>MGACPPKAKGPWAQLQKLLISWPVGEQDWEQYRDRVNMLQQERIRDSPLLQAAKENDLRLLKILLLNQSCDFQQRGAVGETALHVAALYDNLEAATLLMEAAPELAKEPALCEPFVGQTALHIAVMNQNLNLVRALLARGASVSARATGAAFRRSPHNLIYYGEHPLSFAACVGSEEIVRLLIEHGADIRAQDSLGNTVLHILILQPNKTFACQMYNLLLSYDEHSDHLQSLELVPNHQGLTPFKLAGVEGNTVMFQHLMQKRKHVQWTCGPLTSTLYDLTEIDSWGEELSFLELVVSSKKREARQILEQTPVKELVSFKWKKYGRPYFCVLASLYILYMICFTTCCIYRPLKLRDDNRTDPRDITILQQKLLQEAYVTHQDNIRLVGELVTVTGAVIILLLEIPDIFRVGASRYFGQTILGGPFHVIIITYASLVLLTMVMRLTNMNGEVVPLSFALVLGWCSVMYFARGFQMLGPFTIMIQKMIFGDLMRFCWLMAVVILGFASAFHITFQTEDPNNLGEFSDYPTALFSTFELFLTIIDGPANYSVDLPFMYCITYAAFAIIATLLMLNLFIAMMGDTHWRVAQERDELWRAQVVATTVMLERKMPRFLWPRSGICGYEYGLGDRWFLRVENHHDQNPLRVLRYVEAFKCSDKEDGQEQLSEKRPSTVESGMLSRASVAFQTPSLSRTTSQSSNSHRGWEILRRNTLGHLNLGLDLGEGDGEEVYHFTETSQVAPA[4x]

Transient receptor potential vanilloid (TRPV) channels are a group of six polymodal cation channels subdivided into two subgroups by their sequence identity and functional properties. TRPV1–TRPV4 comprise the first subgroup of non-selective Ca2+ channels, TRPV5 and TRPV6 constitute the second subgroup of Ca2+ selective channels. TRPV channels are blocked by ruthenium red (RR), a universal pore blocker for a wide array of cation channels. Here we use cryo-electron microscopy to reveal the molecular details of RR block in TRPV2 and TRPV5, members of the two TRPV subfamilies.

Notably, in our experience the addition of PI(4,5)P2 to TRPV5 consistently yields datasets with a majority of particles with an open lower gate and extra density for PI(4,5)P2 but none similar to the RR in the pore. To determine whether RR occupies the SF in the apo state, we collected a dataset of TRPV5 treated with 1 mM RR, yielding a single state with strong density at the SF with a C4 symmetry at 2.96 Å resolution. The RR molecule in TRPV5RR is coordinated high in the SF, occupying Sites 1 and Site 2. Asp542 forms a polar interaction (3.2 Å) with the top ammonia group (Site 1) and the carbonyl of Thr539 and possibly also the Thr539 sidechain hydroxyl form hydrogen bonds (3.0–3.4 Å) with ammonia groups coordinated with the middle ruthenium atom (Site 2). While the position of RR in TRPV5RR is identical to the position RR occupies in TRPV6, the RR in TRPV5PIP2+RR is positioned notably lower in the SF. Indeed, the structures of both TRPV5RR and TRPV5PIP2+RR are essentially identical to TRPV5Apo, including vanilloid lipid densities, apart from the density for RR. We also observed two possible positions for RR binding in the TRPV5 SF, a higher one which seems to be preferred when the channel has not been opened coordinated at Asp542 and a lower one coordinated by Asn572 which is dominant when the channel has previously been activated by PI(4,5)P2. Yet RR is not tightly coordinated in this position, resulting in somewhat amorphous density. It is not clear how RR enters the TRPV5 pore which is tightly closed at both gates in the TRPV5Apo state. In TRPV5Apo, the lower gate is tightly closed and hydrophobic and the SF is also closed, but provides a favorable environment for the entrance and binding of the positively charged molecule. Therefore, it is most likely that RR enters the TRPV5 pore through the SF, suggesting that the TRPV5 SF may not be not as rigid as commonly accepted.5-BROMOCYTIDINE 5'-(DIHYDROGEN PHOSPHATE) 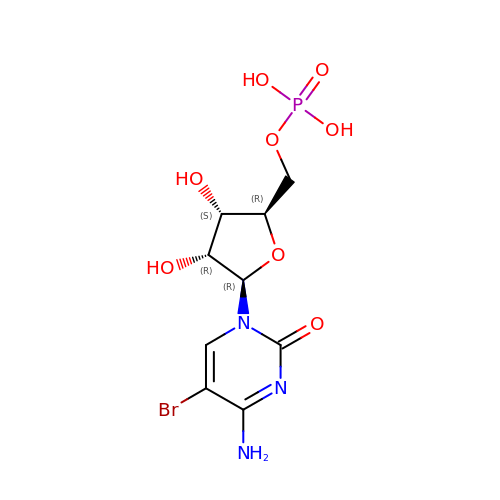| C9 H13 Br N3 O8 P | KOHPTSGPCYTYFB-UAKXSSHOSA-N>[2x]MGPLWGPLYAPVSES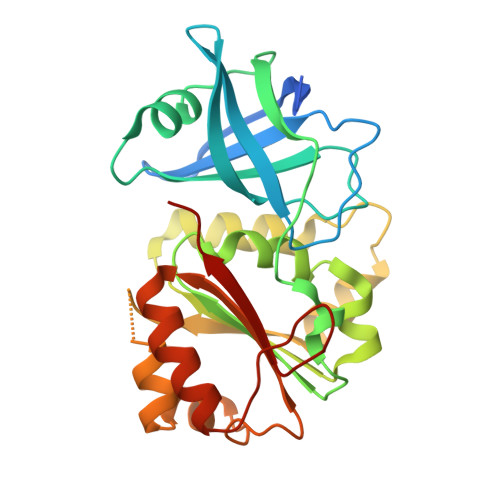MSKFDTATVLSVHHWTDTLFSFTCTRDQALRFNNGEFTMVGLEVDGKPLTRAYSIVSPNYEEHLEFFSIKVQNGPLTSRLQHLKVGDPVLIGKKPTGTLVADNLLPGKTLWMLSTGTGLAPFMSIIRDPDIYERFDKVVLTHTCRLKGELAYMDYIKHDLPGHEYLGDVIREKLVYYPTVTREEFENEGRITDLIASGKLFTDLDMPPFSPEQDRVMLCGSTAMLKDTTELLKKAGLVEGKNSAPGHYVIERAFVD>[6x]M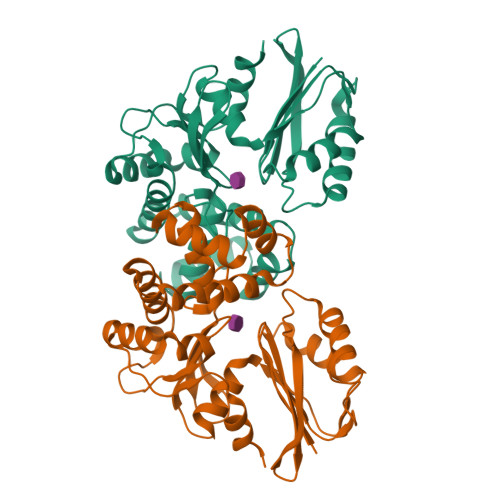AILIADSGSTKTHWNVLDQGRVIGEIFTKGMNPFFQTPEEMGREIERTLLPQLNSNRFCEVHFFGAGCIPEKVPVVRNVLKGCLDVSSLIEVDTDMLAAAKASCGRSPGIVCIMGTGSNSCFYDGEKIAANVSPLGFILGDEGSGAVLGKLLIGDLLKNQMGEELKEKFLRQYELTPANIIERVYRQPFPNRFLAGISPFLAENIEHPAIHSLVLNAFKSFLTRNVMQFDYTRYKAHFIGSVAYYYKDILEEAAAATGIRTGTIVRNPMEGLRTYYSTVAKTVLEHHHHHH>[4x]MGSSHHHHHHHHSSGLVPRGSHLNIYLLPPSSERYGRVILDRVEQRGLYSQGRQWQIIRQRSEKKLKTSKSYQESRNIVQEAVRYGGGKHSQILSKETVRRDTLDSRYPEYRRLNEDILLITIPSISKLDKRSISHYSGKLQNILMEKSYKGLILDLSNNTGGNMIPMIGGLASILPND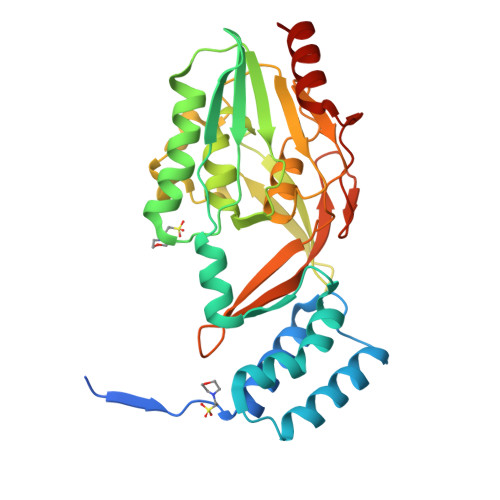TLFHYTDKYGNKKTITMKNIPLEALKISRKTINTKHVPIAIITNHKTASSAEMTFLSFKGLPNVKSFGQATAGYTTVNETFMLYDGARLALTTGIVSDRQGYKYENTPILPDQVTSLPLQESQSWLKSRINQN> KAMAGNFWQSSHYLQWILDKQDLLKERQKDLKFLSEEEYWKLQIFFTNVIQALGEHLKLRQQVIATATVYFKRFYARYSLKSIDPVLMAPTCVFLASKVEEFGVVSNTRLIAAATSVLKTRFSYAFPKEFPYRMNHILECEFYLLELMDCCLIVYHPYRPLLQYVQDMGQEDMLLPLAWRIVND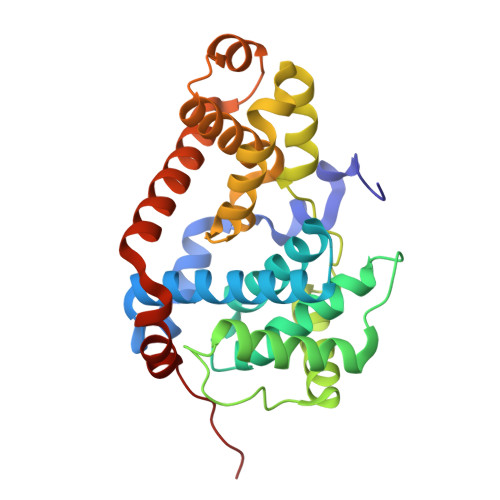TYRTDLCLLYPPFMIALACLHVACVVQQKDARQWFAELSVDMEKILEIIRVILKLYEQWKNFDERKEMATILSKMPKPKPPP>[3x]STNDNIKDL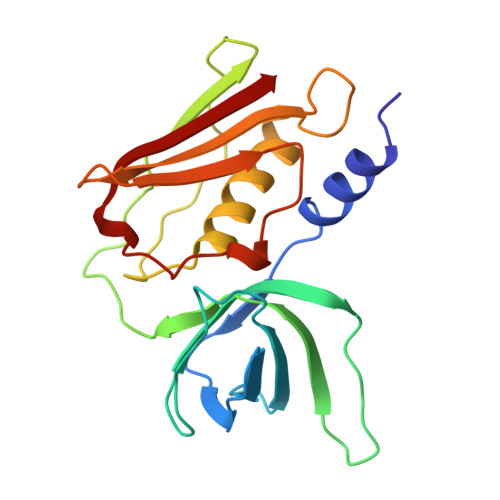LDWYSSGSDTFTNSEVLDNSLGSMRIKNTDGSISLIIFPSPYYSPAFTKGEKVDLNTKRTKKSQHTSEGTYIHFQISGVTNTEKLPTPIELPLKVKVHGKDSPLKYWPKFDKKQLAISTLDFEIRAQLTQIHGLYRSSDKTGGYWKITMNDGSTYQSDLSKKFEYNTEKPPINIDEIKTIEAEIN> MGSDKIHHHHHHENLYFQGMTL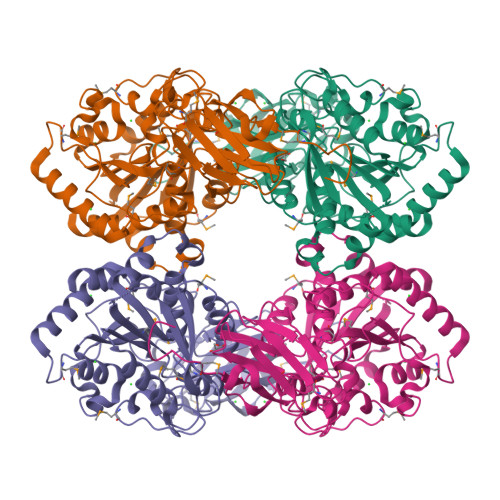SITSNFDAGAIDVVSCERADAIRLRVRGDNRSEFAQWFYFRLTGARGERCVMTFENANDCAYPAGWRDYRAVASYDRVNWFRVPTSYDGQMLTIDHTPEFDSIHYAYFEPYSEERHSEFLGAVQQMPQASVVELGRTVEGRPMSLVVLGTPDEAGAAKKKVWIIARQHPGESMAEWFIEGLVKRLVGWGDWSGDPVARKLYDHATFYIVPNMNPDGSVHGNLRTNAAGANLNREWMEPDAERSPEVLVVRDAIHAIGCDLFFDIHGDEDLPYVFAAGSEMLPGFTEQQRVEQSAFIDSFKRASPDFQDEHGYPPGKYREDAFKLASKYIGHRFGCLSLTLEMPFKDNANLPDEHIGWNGARSASLGAAMLGAILEHVRAFA4-(5-phenyl-1H-pyrrolo[2,3-b]pyridin-3-yl)benzoic acid 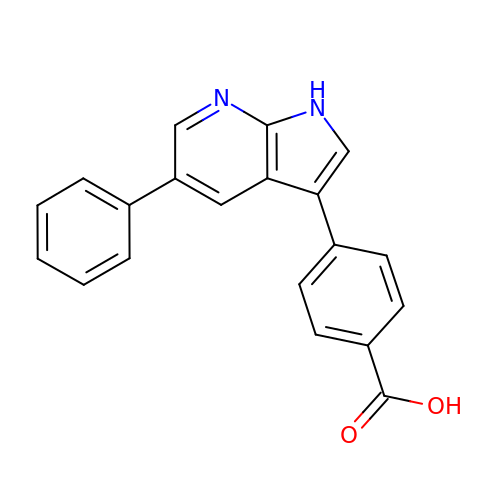| C20 H14 N2 O2 | KSFDVNIKNYXUIP-UHFFFAOYSA-N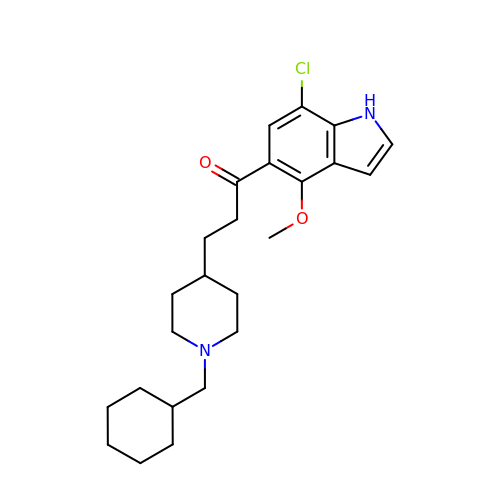1-(7-chloranyl-4-methoxy-1~{H}-indol-5-yl)-3-[1-(cyclohexylmethyl)piperidin-4-yl]propan-1-one | C24 H33 Cl N2 O2 | DUUYHLUSDHATNS-UHFFFAOYSA-N> GGSVEEIRLPRAGGPLGLSIVGGSDHSSHPFGVQEPGVFISKVLPRGLAARSG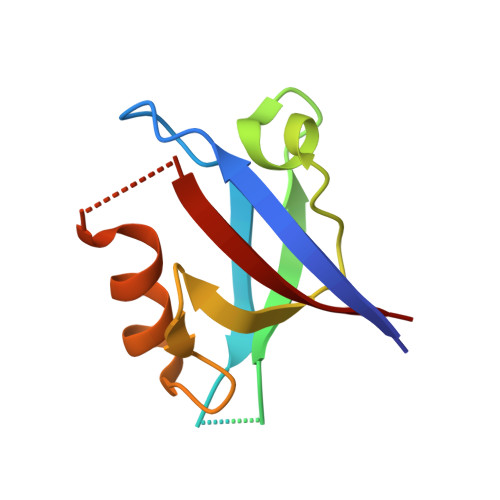LRVGDRILAVNGQDVRDATHQEAVSALLRPCLELSLLVRRD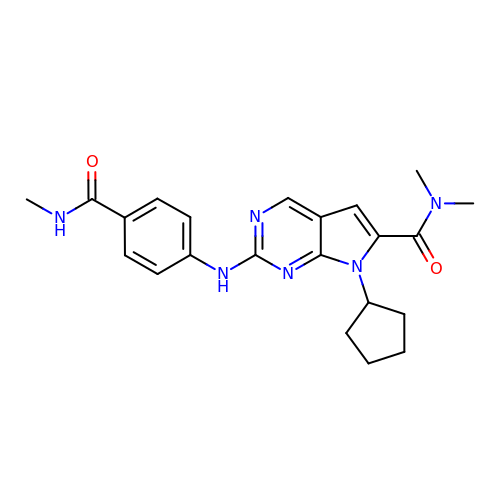7-cyclopentyl-N,N-dimethyl-2-[4-(methylcarbamoyl)anilino]-7H-pyrrolo[2,3-d]pyrimidine-6-carboxamide | C22 H26 N6 O2 | XIUNGGKWWZDBSL-UHFFFAOYSA-N>MLYKEPEDGEKIKFDKGKWIVPNKPVILYIEGDGIGPEITNAAIKVINKAVERAYGSSREIKWLEVYAGEKAEKLVNDRFPKETQEMLLKYRVVLKGPLETPIGKGWKSVNVAIRLMLDLYANIRPVKYIEGLESPLKHPEKVDMIIFRENTDDLYRGIEYPFNSEEAKKIRDFLRKELKVEIEDDTGIGIKVMSKYKTQRITRLAIQYAIEHKRKKVTIMHKGNVMKYTEGAFREWAYEVALKEYRDFIVTEEEINQGKPDQGKIILNDRIADNMFQQIIIRPEEYDIILAPNVNGDYISDAAGALIGNIGMLGGANIGDEGGMFEAIHGTAPKYAGKNVANPTGIIKAGELMLRWMGWNEAADLIEKAINMAIRDKKVTQDIARFMGVKALGTKEYADELIKIMDTI[2x]

Isocitrate dehydrogenase (IDH) catalyzes the oxidative decarboxylation of isocitrate to produce α-ketoglutarate and CO2 while reducing the cofactor nicotinamide adenine dinucleotide (phosphate) (NAD(P)+) to NAD(P)H using divalent metal cation (Mg2+ or Mn2+) in the tricarboxylic acid cycle. Although the amino acid sequence identity between subfamilies I and II is low (<20%), both IDHs function as homodimers; each monomer is composed of three domains: large, small, and clasp domains, and the active site is situated between the large and small domains. The thermoacidophilic archaeon Sulfolobus tokodaii strain 7, which grows optimally at 75°C and pH 3, has an open reading frame ST2166 in the genome encoding hypothetical IDH. In this study, we expressed, purified, and determined the crystal structures of ST2166 in the apo and NADP+-bound forms at 2.0 Å and 2.4 Å resolutions, respectively, and discussed the mechanisms for cofactor recognition of prokaryotic NADP-IDHs.

When the apo crystals were soaked with NADP+, ST2166 could bind NADP+ within the active site without conformational changes with RMSD of 0.19 Å for 401 Cα atoms between those in the apo and NADP+-bound (holo) forms. The crystal structure in complex with NADP+ contains 403 amino acid residues (residues 103–108 are disordered) per subunit, NADP+, and 405 water molecules. NADP+ is bound with the residues derived from the large domain at the upper part of the open active site cleft, apart from the postulated isocitrate-binding site, suggesting that the substrate access to its binding site may not be limited. The electron density maps clearly revealed that the NADP+ molecule adopts a U-shaped conformation, in which the adenine ring and the nicotinamide ring are in the anticonformation with respect to each adjacent ribose. The adenine ring is hydrogen bonded with the main chain oxygen of Asn343 in the Dj loop (N6A–O). In the deep cleft, the nicotinamide ring interacts with the side chains of Asn111 in the Cd loop (O7N–ND2) and Glu327 in the carboxyl terminal of the D strand (N7N–OE1) and with the main chain of Leu99 in the C strand (O7N–N/O). The adjacent ribose is hydrogen bonded to the side chain of Glu100 (O3D-OE1) and the main chain nitrogen of Thr101 (O2D–N) both in the Cd loop. The 2′-phosphate group of NADP+ is bound to the side chains of Lys335 (OP3–NZ), Tyr336 (OP2–OH), and Arg386 (OP2–NH1). Because NAD+ possesses a hydroxyl group at the 2′-moiety, these direct interactions of the large domain with the 2′-phosphate group of NADP+ from a single subunit are responsible for the discrimination of NADP+ from NAD as a cofactor in the open form of ST2166. Therefore, it is conceivable that the cofactor selectivity in prokaryote NADP-IDHs is determined by the three residues Lys335, Tyr336, and Arg386 in ST2166 binding to the 2′-phosphate group of NADP+ in the open form, not in the closed form.Phosphoketolase (XPK) belongs to the transketolase family, a member of thiamine pyrophosphate (TPP)-dependent enzyme superfamily. It converts F6P, xylulose-5-phosphate (Xu5P) or sedoheptulose-7-phosphate (S7P), which are intermediates in RuBP regeneration, to produce acetyl phosphate (AcP) and C3, C4 or C5 sugar phosphates. XPK is an enzyme present in many microorganisms, primarily involved in substrate-level phosphorylation to produce AcP.

On the other hand, Bifidobacterium longum XPK showed no inhibition by ATP. Comparison between the C-terminal interfaces of free SeXPK and free B. longum XPK structures provides a structural basis for the lack of ATP inhibition in B. longum XPK.

>[2x]MTSPVIGTPWKKLNAPVSEEALEGVDKYWRVANYLSIGQIYLRSNPLMKEPFTREDVKHRLVGHWGTTPGLNFLIGHINRFIADHGQNTVIIMGPGHGGPAGTSQSYLDGTYTETFPKITKDEAGLQKFFRQFSYPGGIPSHFAPETPGSIHEGGELGYALSHAYGAIMDNPSLFVPAIVGDGEAETGPLATGWQSNKLVNPRTDGIVLPILHLNGYKIANPTILSRISDEELHEFFHGMGYEPYEFVAGFDDEDHMSIHRRFAELWETIWDEICDIKATAQTDNVHRPFYPMLIFRTPKGWTCPKYIDGKKTEGSWRSHQVPLASARDTEAHFEVLKNWLESYKPEELFDANGAVKDDVLAFMPKGELRIGANPNANGGVIRNDLKLPNLEDYEVKEVAEYGHGWGQLEATRTLGAYTRDIIKNNPRDFRIFGPDETASNRLQASYEVTNKQWDAGYISDEVDEHMHVSGQVVEQLSEHQMEGFLEAYLLTGRHGIWSSYESFVHVIDSMLNQHAKWLEATVREIPWRKPIASMNLLVSSHVWRQDHNGFSHQDPGVTSVLLNKCFHNDHVIGIYFATDANMLLAIAEKCYKSTNKINAIIAGKQPAATWLTLDEARAELEKGAAAWDWASTAKNNDEAEVVLAAAGDVPTQEIMAASDKLKELGVKFKVVNVADLLSLQSAKENDEALTDEEFADIFTADKPVLFAYHSYAHDVRGLIYDRPNHDNFNVHGYEEEGSTTTPYDMVRVNRIDRYELTAEALRMIDADKYADKIDELEKFRDEAFQFAVDNGYDHPDYTDWVYSGVNTDKKGAVTATAATAGDNE> MIEEHNCFEEFINTAAIGEQQVYGEYKSKLDSFTDESKLPYELLLERKNLVELKISDEEYKKSESALKTPNPTLLQKFQINFYQTIESINQVFKPSSSSSNQSSSSSSSNEDDSLQNKKIKVMSWHPQHRLLAVCNKNDVIYIYYFPNQDMYGMGNVRPLTLWFELQSKVYDIQWKPFLPYTLAVACENGIILWEIDISDLKVELKRTSPNYRINQSSTCANILNYPYFLSNTITWSSNGLQLACGSTNHSSILLWDVVSRVPTFIPRYN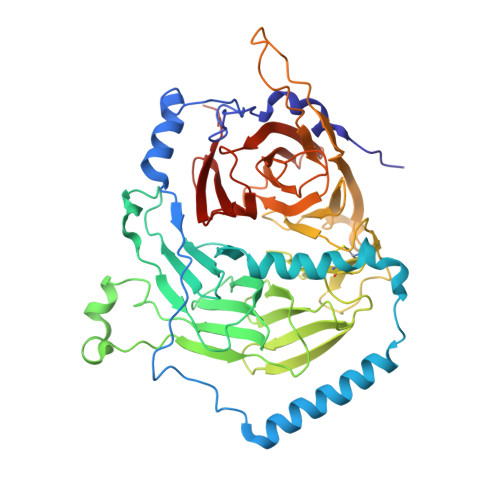GNSLLVWSPKNDYLLSCGGKTCRIFDISKWDYNNKEWPMLTNYQTGSWNGKGEYLAVASGDRIQFIQCINRAFESGGELMYVEKTSTYRLQNVGGSGGGSSSSELFLGGHIKKIAWSPDSQRLAVIFYLNSKSRNNDTYCAIYKIKTYPKFSVTPRGFIRSKDQSIQSVSFVPNYKKGSLLSIAYNDGTIKFFPLLYQYKQ> VPAAVDWRTAGAVTPVKNQQQCGCCWAFSAVAAIEGATQIKTGTLTSLSEEQIVDCDTNGNDKGCNGGTPDGAFQYVVNNQGIDTESDYPYTAGGGSPGTCSASSYQPAASITGYQDVPANNEQALQQAAATQPISVAIDASDPSFQS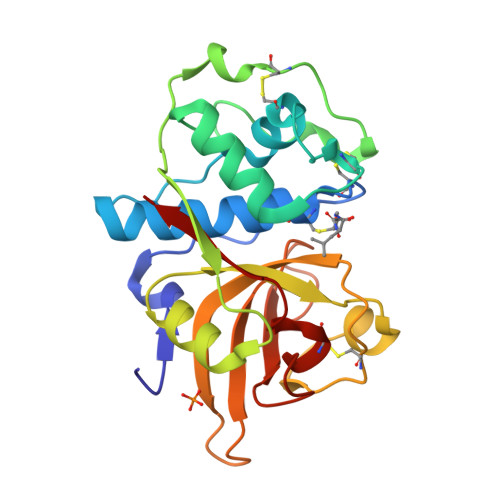YSSGIYSGPCNTNLDHAVTVVGYGTDPNSGNSYWIVKNSWGTSWGQEGYIWMQMGLNAPYGVCGIAMQASYPTA>MKSSELNQRRQQATPRGVGVMCNYFVEKAENATLWDIEGNEVIDFAAGIAVLNTGHRHPKVVAAVADQLQAFTHTAYQIVPYESYVSLAERINDLAPIDGPAKTAFFTTGAEAVENAVK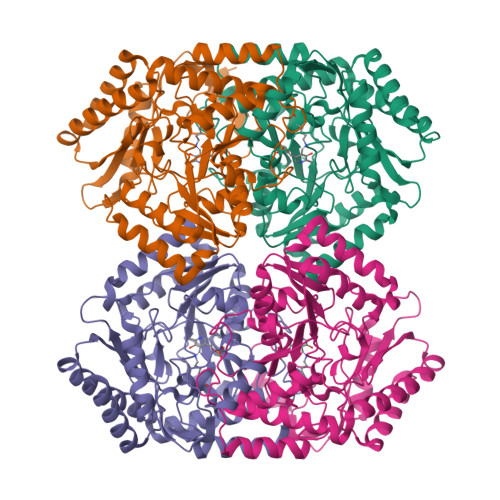IARAYTGRPGLITFGGGFHGRTFMTMALTGKVAPYKIGFGPFPGSVYHGVYPNAAHGVTTADALKSLERIFKADIAPDQVAAIILEPIQGEGGFNVAPADFMQALRDLCDTHGILLIADEVQTGFARTGKLFAMQHYEVKPDLMTMAKSLAGGFPLSGVVGRAEVMDAPAPGGLGGTYAGNPLAVAAAHAVLDVIAEEQLCQRAEQLGSHLQEVLNQARATCPAIVDVRGRGSMVAVEFNDPQTGEPSPEFTRLVQQKAQENGLLLLSCGVYGNVIRFLYPLTIPDAQFSKALDILARVLKS[4x]>MEDEIRKAAEILAKSKHAVVFTGAGISAESGIPTFRGEDGLWRKYDPEEVASISGFKRNPRAFWEFSMEMKDKLFAEPNPAHYAIAELERMGIVKAVITQNIDMLHQRAGSRRVLELHGSMDKLDCLDCHETY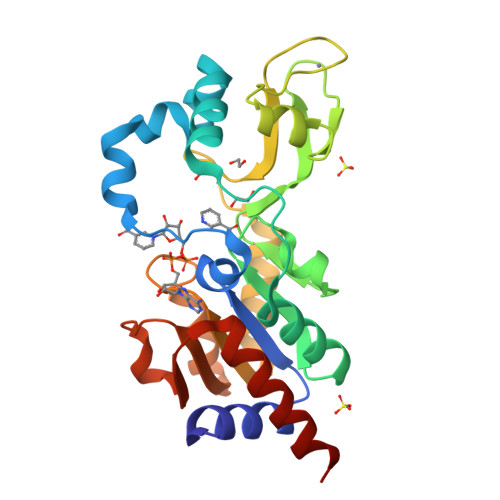DWSEFVEDFNKGEIPRCRKCGSYYVKPRVVLFGEPLPQRTLFEAIEEAKHCDAFMVVGSSLVVYPAAELPYIAKKAGAKMIIVNAEPTMADPIFDVKIIGKAGEVLPKIVEEVKRLRSEK[5x]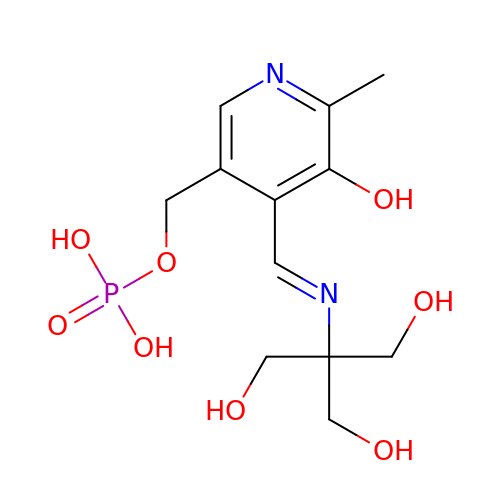[4-[[[2-(hydroxymethyl)-1,3-bis(oxidanyl)propan-2-yl]amino]methyl]-6-methyl-5-oxidanyl-pyridin-3-yl]methyl dihydrogen phosphate | C12 H19 N2 O8 P | GKGTZXISICTHPS-LZWSPWQCSA-N>MEEIYAKFVSQKISKTRWRPLPPGSLQTAETFATGSWDNEENYISLWSIGDFGNLDSDGGFEGDHQLLCDIRHHGDVMDLQFFDQERIVAASSTGCVTVFLHHPNNQTLSVNQQWTTAHYHTGPGSPSYSSAPCTGVVCNNPEIVTVGEDGRINLFRADHKEAVRTIDNADSSTLHAVTFLRTPEILTVNSIGQLKIWDFRQQGNEPSQILSLTGDRVPLHCVDRHPNQQHVVATGGQDGMLSIWDVRQGTMPVSLLKAHEAEMWEVHFHPSNPEHLFTCSEDGSLWHWDASTDVPEKSSLFHQGGRSSTFLSHSISNQANVHQSVISSWLSTDPAKDRIEITSLLPSRSLSVNTLDVLGPCLVCGTDAEAIYVTRHLFS[4x];>[4x]MLHLSAAPPAPPPEVTATARPCLCSVGRRGDGGKMAAAGALERSFVELSGAERERPRHFREFTVCSIGTANAVAGAVKYSESAGGFYYVESGKLFSVTRNRFIHWKTSGDTLELMEESLDINLLNNAIRLKFQNCSVLPGGVYVSETQNRVIILMLTNQTVHRLLLPHPSRMYRSELVVDSQMQSIFTDIGKVDFTDPCNYQLIPAVPGISPNSTASTAWLSSDGEALFALPCASGGIFVLKLPPYDIPGMVSVVELKQSSVMQRLLTGWMPTAIRGDQSPSDRPLSLAVHCVEHDAFIFALCQDHKLRMWSYKEQMCLMVADMLEYVPVKKDLRLTAGTGHKLRLAYSPTMGLYLGIYMHAPKRGQFCIFQLVSTESNRYSLDHISSLFTSQETLIDFALTSTDIWALWHDAENQTVVKYINFEHNVAGQWNPVFMQPLPEEEIVIRDDQDPREMYLQSLFTPGQFTNEALCKALQIFCRGTERNLDLSWSELKKEVTLAVENELQGSVTEYEFSQEEFRNLQQEFWCKFYACCLQYQEALSHPLALHLNPHTNMVCLLKKGYLSFLIPSSLVDHLYLLPYENLLTEDETTISDDVDIARDVICLIKCLRLIEESVTVDMSVIMEMSCYNLQSPEKAAEQILEDMITIDVENVMEDICSKLQEIRNPIHAIGLLIREMDYETEVEMEKGFNPAQPLNIRMNLTQLYGSNTAGYIVCRGVHKIASTRFLICRDLLILQQLLMRLGDAVIWGTGQLFQAQQDLLHRTAPLLLSYYLIKWGSECLATDVPLDTLESNLQHLSVLELTDSGALMANRFVSSPQTIVELFFQEVARKHIISHLFSQPKAPLSQTGLNWPEMITAITSYLLQLLWPSNPGCLFLECLMGNCQYVQLQDYIQLLHPWCQVNVGSCRFMLGRCYLVTGEGQKALECFCQAASEVGKEEFLDRLIRSEDGEIVSTPRLQYYDKVLRLLDVIGLPELVIQLATSAITEAGDDWKSQATLRTCIFKHHLDLGHNSQAYEALTQIPDSSRQLDCLRQLVVVLCERSQLQDLVEFPYVNLHNEVVGIIESRARAVDLMTHNYYELLYAFHIYRHNYRKAGTVMFEYGMRLGREVRTLRGLEKQGNCYLAALNCLRLIRPEYAWIVQPVSGAVYDRPGASPKRNHDGECTAAPTNRQIEILELEDLEKECSLARIRLTLAQHDPSAVAVAGSSSAEEMVTLLVQAGLFDTAISLCQTFKLPLTPVFEGLAFKCIKLQFGGEAAQAEAWAWLAANQLSSVITTKESSATDEAWRLLSTYLERYKVQNNLYHHCVINKLLSHGVPLPNWLINSYKKVDAAELLRLYLNYDLLEEAVDLVSEYVDAVLGKGHQYFGIEFPLSATAPMVWLPYSSIDQLLQALGENSANSHNIALSQKILDKLEDYQQKVDKATRDLLYRRTL;>MKQDASRNAAYTVDCEDYVHVVEFNPFENGDSGNLIAYGGNNYVVIGTCTFQEEEADVEGIQYKTLRTFHHGVRVDGIAWSPETRLDSLPPVIKFCTSAADMKIRLFTSDLQDKNEYKVLEGHTDFINGLVFDPKEGQEIASVSDDHTCRIWNLEGVQTAHFVLHSPGMSVCWHPEETFKLMVAEKNGTIRFYDLLAQQAILSLESEQVPLMSAHWCLKNTFKVGAVAGNDWLIWDITRSSYPQNKRPVHMDRACLFRWSTISENLFATTGYPGKMASQFQIHHLGHPQPILMGSVAVGSGLSWHRTLPLCVIGGDHKLLFWVTEV[4x];>[4x]MFPAAPSPRTPGTGSRRGPLAGLGPGSTPRTASRKGLPLGSAVSSPVLFSPVGRRSSLSSRGTPTRMFPHHSITESVNYDVKTFGSSLPVKVMEALTLAEVDDQLTINIDEGGWACLVCKEKLIIWKIALSPITKLSVCKELQLPPSDFHWSADLVALSYSSPSGEAHSTQAVAVMVATREGSIRYWPSLAGEDTYTEAFVDSGGDKTYSFLTAVQGGSFILSSSGSQLIRLIPESSGKIHQHILPQGQGMLSGIGRKVSSLFGILSPSSDLTLSSVLWDRERSSFYSLTSSNISKWELDDSSEKHAYSWDINRALKENITDAIWGSESNYEAIKEGVNIRYLDLKQNCDGLVILAAAWHSADNPCLIYYSLITIEDNGCQMSDAVTVEVTQYNPPFQSEDLILCQLTVPNFSNQTAYLYNESAVYVCSTGTGKFSLPQEKIVFNAQGDSVLGAGACGGVPIIFSRNSGLVSITSRENVSILAEDLEGSLASSVAGPNSESMIFETTTKNETIAQEDKIKLLKAAFLQYCRKDLGHAQMVVDELFSSHSDLDSDSELDRAVTQISVDLMDDYPASDPRWAESVPEEAPGFSNTSLIILHQLEDKMKAHSFLMDFIHQVGLFGRLGSFPVRGTPMATRLLLCEHAEKLSAAIVLKNHHSRLSDLVNTAILIALNKREYEIPSNLTPADVFFREVSQVDTICECLLEHEEQVLRDAPMDSIEWAEVVINVNNILKDMLQAASHYRQNRNSLYRREESLEKEPEYVPWTATSGPGGIRTVIIRQHEIVLKVAYPQADSNLRNIVTEQLVALIDCFLDGYVSQLKSVDKSSNRERYDNLEMEYLQKRSDLLSPLLSLGQYLWAASLAEKYCDFDILVQMCEQTDNQSRLQRYMTQFADQNFSDFLFRWYLEKGKRGKLLSQPISQHGQLANFLQAHEHLSWLHEINSQELEKAHATLLGLANMETRYFAKKKTLLGLSKLAALASDFSEDMLQEKIEEMAEQERFLLHQETLPEQLLAEKQLNLSAMPVLTAPQLIGLYICEENRRANEYDFKKALDLLEYIDEEEDININDLKLEILCKALQRDNWSSSDGKDDPIEVSKDSIFVKILQKLLKDGIQLSEYLPEVKDLLQADQLGSLKSNPYFEFVLKANYEYYVQGQI;>MDRSGFGEISSPVIREAEVTRTARKQSAQKRVLLQASQDENFGNTTPRNQVIPRTPSSFRQPFTPTSRSLLRQPDISCILGTGGKSPRLTQSSGFFGNLSMVTNLDDSNWAAAFSSQRSGLFTNTEPHSITEDVTISAVMLREDDPGEAASMSMFSDFLQSFLKHSSSTVFDLVEEYENICGSQVNILSKIVSRATPGLQKFSKTASMLWLLQQEMVTWRLLASLYRDRIQSALEEESVFAVTAVNASEKTVVEALFQRDSLVRQSQLVVDWLESIAKDEIGEFSDNIEFYAKSVYWENTLHTLKQRQLTSYVGSVRPLVTELDPDAPIRQKMPLDDLDREDEVRLLKYLFTLIRAGMTEEAQRLCKRCGQAWRAATLEGWKLYHDPNVNGGTELEPVEGNPYRRIWKISCWRMAEDELFNRYERAIYAALSGNLKQLLPVCDTWEDTVWAYFRVMVDSLVEQEIQTSVATLDETEELPREYLGANWTLEKVFEELQATDKKRVLEENQEHYHIVQKFLILGDIDGLMDEFSKWLSKSRNNLPGHLLRFMTHLILFFRTLGLQTKEEVSIEVLKTYIQLLIREKHTNLIAFYTCHLPQDLAVAQYALFLESVTEFEQRHHCLELAKEADLDVATITKTVVENIRKKDNGEFSHHDLAPALDTGTTEEDRLKIDVIDWLVFDPAQRAEALKQGNAIMRKFLASKKHEAAKEVFVKIPQDSIAEIYNQCEEQGMESPLPAEDDNAIREHLCIRAYLEAHETFNEWFKHMNSVPQKPALIPQPTFTEKVAHEHKEKKYEMDFGIWKGHLDALTADVKEKMYNVLLFVDGGWMVDVREDAKEDHERTHQMVLLRKLCLPMLCFLLHTILHSTGQYQECLQLADMVSSERHKLYLVFSKEELRKLLQKLRESSLMLLDQGLDPLGYEIQL[4x];>SKYGLQDSDEEEEEHPSKTSTKKLKTAPLPPASQTTPLQMALNGKPAPPPQSQSPEVEQLGRVVELDSDMVDITQEPVLDTMLEESMPEDQEPVSASTHIASSLGINPHVLQIMKASLLTDEEDVDMALDQRFSRLPSKADTSQEICSPRLPISASHSSKTRSLVGGLLQ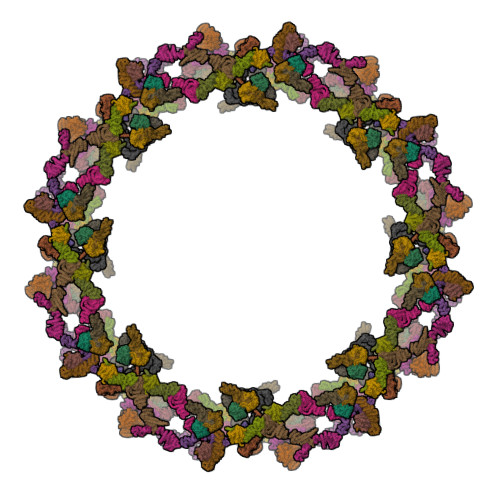SKFTSGAFLSPSVSVQECRTPRAASLMNIPSTSSWSVPPPLTSVFTMPSPAPEVPLKTVGTRRQLGLVPREKSVTYGKGKLLMDMALFMGRSFRVGWGPNWTLANSGEQLNGSHELENHQIADSMEFGFLPNPVAVKPLTESPFKVHLEKLSLRQRKPDEDMKLYQTPLELKLKHSTVHVDELCPLIVPNLGVAVIHDYADWVKEASGDLPEAQIVKHWSLTWTLCEALWGHLKELDSQLNEPREYIQILERRRAFSRWLSCTATPQIEEEVSLTQKNSPVEAVFSYLTGKRISEACSLAQQSGDHRLALLLSQFVGSQSVRELLTMQLVDWHQLQADSFIQDERLRIFALLAGKPVWQLSEKKQINVCSQLDWKRSLAIHLWYLLPPTASISRALSMYEEAFQNTSDSDRYACSPLPSYLEGSGCVIAEEQNSQTPLRDVCFHLLKLYSDRHYDLNQLLEPRSITADPLDYRLSWHLWEVLRALNYTHLSAQCEGVLQASYAGQLESEGLWEWAIFVLLHIDNSGIREKAVRELLTRHCQLLETPESWAKETFLTQKLRVPAKWIHEAKAVRAHMESDKHLEALCLFKAEHWNRCHKLIIRHLASDAIINENYDYLKGFLEDLAPPERSSLIQDWETSGLVYLDYIRVIEMLRHIQQVDCSGNDLEQLHIKVTSLCSRIEQIQCYSAKDRLAQSDMAKRVANLLRVVLSLHHPPDRTSDSTPDPQRVPLRLLAPHIGRLPMPEDYAMDELRSLTQSYLRELAVGSL[4x];>[4x]MVSVINTVDTSHEDMIHDAQMDYYGTRLATCSSDRSVKIFDVRNGGQILIADLRGHEGPVWQVAWAHPMYGNILASCSYDRKVIIWREENGTWEKSHEHAGHDSSVNSVCWAPHDYGLILACGSSDGAISLLTYTGEGQWEVKKINNAHTIGCNAVSWAPAVVPGSLIDHPSGQKPNYIKRFASGGCDNLIKLWKEEEDGQWKEEQKLEAHSDWVRDVAWAPSIGLPTSTIASCSQDGRVFIWTCDDASSNTWSPKLLHKFNDVVWHVSWSITANILAVSGGDNKVTLWKESVDGQWVCISDVNKGQGSVSASVTEGQQNEQ;>MFVARSIAADHKDLIHDVSFDFHGRRMATCSSDQSVKVWDKSESGDWHCTASWKTHSGSVWRVTWAHPEFGQVLASCSFDRTAAVWEEIVGESNDKLRGQSHWVKRTTLVDSRTSVTDVKFAPKHMGLMLATCSADGIVRIYEAPDVMNLSQWSLQHEISCKLSCSCISWNPSSSRAHSPMIAVGSDDSSPNAMAKVQIFEYNENTRKYAKAETLMTVTDPVHDIAFAPNLGRSFHILAIATKDVRIFTLKPVRKELTSSGGPTKFEIHIVAQFDNHNSQVWRVSWNITGTVLASSGDDGCVRLWKANYMDNWKCTGILKGNGSPVNGSSQQGTSNPSLGSTIPSLQNSLNGSSAGRKHS[4x];>[4x]MEELDGEPTVTLIPGVNSKKNQMYFDWGPGEMLVCETSFNKKEKSEMVPSCPFIYIIRKDVDVYSQILRKLFNESHGIFLGLQRIDEELTGKSRKSQLVRVSKNYRSVIRACMEEMHQVAIAAKDPANGRQFSSQVSILSAMELIWNLCEILFIEVAPAGPLLLHLLDWVRLHVCEVDSLSADVLGSENPSKHDSFWNLVTILVLQGRLDEARQMLSKEADASPASAGICRIMGDLMRTMPILSPGNTQTLTELELKWQHWHEECERYLQDSTFATSPHLESLLKIMLGDEAALLEQKELLSNWYHFLVTRLLYSNPTVKPIDLHYYAQSSLDLFLGGESSPEPLDNILLAAFEFDIHQVIKECSIALSNWWFVAHLTDLLDHCKLLQSHNLYFGSNMREFLLLEYASGLFAHPSLWQLGVDYFDYCPELGRVSLELHIERIPLNTEQKALKVLRICEQRQMTEQVRSICKILAMKAVRNNRLGSALSWSIRAKDAAFATLVSDRFLRDYCERGCFSDLDLIDNLGPAMMLSDRLTFLGKYREFHRMYGEKRFADAASLLLSLMTSRIAPRSFWMTLLTDALPLLEQKQVIFSAEQTYELMRCLEDLTSRRPVHGESDTEQLQDDDIETTKVEMLRLSLARNLARAIIREGSLEGS;>MPSSLLGAAMPASTSAAALQEALENAGRLIDRQLQEDRMYPDLSELLMVSAPNNPTVSGMSDMDYPLQGPGLLSVPNLPEISSIRRVPLPPELVEQFGHMQCNCMMGVFPPISRAWLTIDSDIFMWNYEDGGDLAYFDGLSETILAVGLVKPKAGIFQPHVRHLLVLATPVDIVILGLSYANLQTGSGVLNDSLSGGMQLLPDPLYSLPTDNTYLLTITSTDNGRIFLAGKDGCLYEVAYQAEAGWFSQRCRKINHSKSSLSFLVPSLLQFTFSEDDPILQIAIDNSRNILYTRSEKGVIQVYDLGQDGQGMSRVASVSQNAIVSAAGNIARTIDRSVFKPIVQIAVIENSESLDCQLLAVTHAGVRLYFSTCPFRQPLARPNTLTLVHVRLPPGFSASSTVEKPSKVHRALYSKGILLMAASENEDNDILWCVNHDTFPFQKPMMETQMTAGVDGHSWALSAIDELKVDKIITPLNKDHIPITDSPVVVQQHMLPPKKFVLLSAQGSLMFHKLRPVDQLRHLLVSNVGGDGEEIERFFKLHQEDQACATCLILACSTAACDREVSAWATRAFFRYGGEAQMRFPTTLPPPSNVGPILGSPVYSSSPVPSGSPYPNPSFLGTPSHGIQPPAMSTPVCALGNPATQATNMSCVTGPEIVYSGKHNGICIYFSRIMGNIWDASLVVERIFKSGNREITAIESSVPCQLLESVLQELKGLQEFLDRNSQFAGGPLGNPNTTAKVQQRLIGFMRPENGNPQQMQQELQRKFHEAQLSEKISLQAIQQLVRKSYQALALWKLLCEHQFTIIVAELQKELQEQLKITTFKDLVIRDKELTGALIASLINCYIRDNAAVDGISLHLQDICPLLYSTDDAICSKANELLQRSRQVQNKTEKERMLRESLKEYQKISNQVDLSNVCAQYRQVRFYEGVVELSLTAAEKKDPQGLGLHFYKHGEPEEDIVGLQAFQERLNSYKCITDTLQELVNQSKAAPQSPSVPKKPGPPVLSSDPNMLSNEEAGHHFEQMLKLSQRSKDELFSIALYNWLIQVDLADKLLQVASPFLEPHLVRMAKVDQNRVRYMDLLWRYYEKNRSFSNAARVLSRLADMHSTEISLQQRLEYIARAILSAKSSTAISSIAADGEFLHELEEKMEVARIQLQIQETLQRQYSHHSSVQDAVSQLDSELMDITKLYGEFADPFKLAECKLAIIHCAGYSDPILVQTLWQDIIEKELSDSVTLSSSDRMHALSLKIVLLGKIYAGTPRFFPLDFIVQFLEQQVCTLNWDVGFVIQTMNEIGVPLPRLLEVYDQLFKSRDPFWNRMKKPLHLLDCIHVLLIRYVENPSQVLNCERRRFTNLCLDAVCGYLVELQSMSSSVAVQAITGNFKSLQAKLERLH[2x]7-hydroxy-4-methyl-2H-chromen-2-one | C10 H8 O3 | 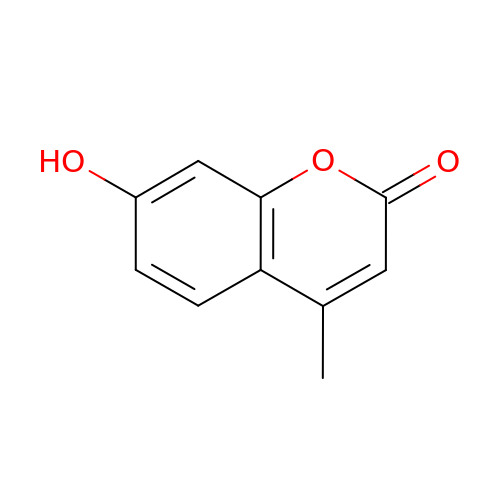HSHNITRMYYLLCV-UHFFFAOYSA-N>MELHILEHRVRVLSVARPGLWLYTHPLIKLLFLPRRSRCKFFSLTETPEDYTLMVDEEGFKELPPSEFLQVAEATWLVLNVSSHSGAAVQAAGVTKIARSVIAPLAEHHVSVLMLSTYQTDFILVREQDLSVVIHTLAQEFDIYREVGGEPVPVTRDDSSNGFPRTQHGPSPTVHPIQSPQNRFCVLTLDPETLPAIATTLIDVLFYSHSTPKEAASSSPEPSSITFFAFSLIEGYISIVMDAETQKKFPSD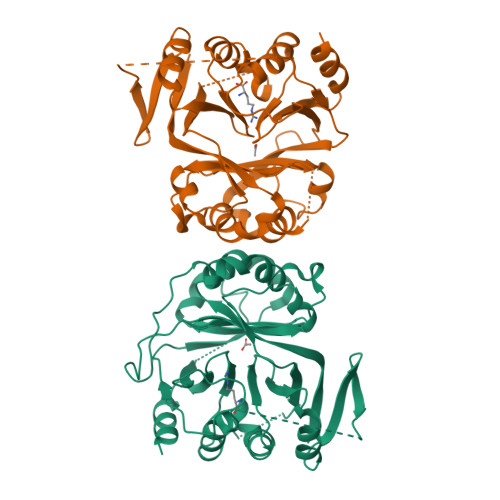LLLTSSSGELWRMVRIGGQPLGFDECGIVAQIAGPLAAADISAYYISTFNFDHALVPEDGIGSVIEVLQRRQEGLAS[4x]> MYMKKLVFGGMLIVSAASLVGCMSQIGSSVRQAVSDNQSAQTLVEWENSEANPEALFANWRHEFMVDSSKRESMKTELCKELQALPAQDLTLFENEIRDENNRALVSGCKEELLAQVDEHFDEQRESMSVPGHALKAVQSRNSFRFPDNTQKRDMSNGYMAVRGDVARKEVVLTFDDGPHGLYTDAILRALKEVNAKAMFFATGKSVRTNPEALKRVAADGHVIGSHSITHACLGTSVACYKQMGNRNLTFDEAAAEVRGGHQAVFDVLGWVDPVFRFXYGETSKDLKAFLKTKSTGEFAWNIESDDWRTQSNEQLLARVLANVESQGRGIVLFHDIQRRTAEIMPQFLRELYNRGYSVVLLTAADPSAKYNSKLVKRKQQLP

Bdellovibrio bacteriovorus is a small predatory bacterium which enters the periplasm of Gram-negative prey cells forming a transient structure called a bdelloplast. We identified two related genes (bd0468 and bd3279) in the B. bacteriovorus HD100 genome whose products had homology to one domain of the peptidoglycan deacetylase PgdA of Streptococcus pneumoniae. Here we show that both genes are expressed early in predation and act upon the GlcNAc residues of the prey cell to modify the prey peptidoglycan structure. In contrast to early ideas of solely stabilising prey peptidoglycan; the modification caused by the Bd0468 and Bd3279 GlcNAc deacetylases targets the prey bdelloplast peptidoglycan for destruction at the end of the predatory cycle, and without it a “ghost” of prey- bacterial peptidoglycan and some membrane remains after Bdellovibrio predation.

We obtained a high-resolution structure of the secreted, mature form of Bd3279 (encompassing amino acids 24–383) at 1.5 Å resolution. Bd3279 is comprised of two domains, an N-terminal domain (NTD, amino acids 24–126) and the catalytic C-terminal domain (CTD, amino acids 127–383). The NTD forms a compact structure comprised of seven regular and two 310 α-helices, stabilized by a disulphide bond between residues Cys79 and Cys109. This domain approximately resembles a “cap” over the active site of the enzyme, and has no precedent in existing peptidoglycan deacetylase protein structures; indeed, the sequence of this region appears to be unique to Bdellovibrio and its close relatives. One of the active site loops of Bd3279 is at least partially disordered, with weak electron density for amino acids 229/230 and no interpretable electron density for region 231–248. The CE-4 ×2+ catalytic ion binding pocket is present in Bd3279, co-ordinated by residues His227 and Asp177; the third superfamily-conserved ion liganding residue would be expected to be contributed by His231, which is present in the disordered active site loop and thus not modelled in our structure. In-line with homologous CE-4 domains, we have modelled the ion as Zn2+, putatively arising from co-purification as no exogenous zinc was added at any stage. Unique to Bd3279, the NTD sits over these active site motifs, with residues Leu43, Val44, Trp46 and Glu47 projecting into the substrate-binding cleft; such proximity may regulate enzyme activity. In total, the structure of Bd3279 confirms that deacetylase activity is likely to be attributable to the same conserved machinery of other, previously characterized CE-4 enzymes, but with unique flanking features (obscuring of substrate binding cleft by novel N-terminal domain “plugging”; extension of active site by disordered loop) that currently appear to be predator-specific. Domain closure appears to have affected the position of two active site motifs, given that His231 and Tyr280 are in orientations incompatible with catalysis, yet we observe activity with the purified protein.>[2x]GSMSEQSICQARAAVMVYDDANKKWVPAGGSTGFSRVHIYHHTGNNTFRVVGRKIQDHQVVINCAIPKGLKYNQATQTFHQWRDARQVYGLNFGSKEDANVFASAMM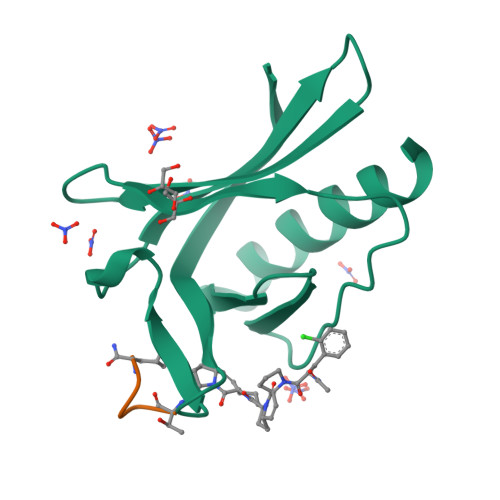HALEVL;>TEDEL[2x]3-Dehydrosphinganine 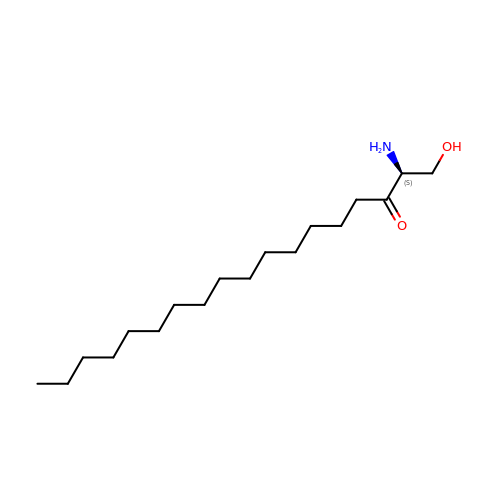| C18 H37 N O2 | KBUNOSOGGAARKZ-KRWDZBQOSA-N Family VIII esterases present similarities to class C β‐lactamases, which show nucleophilic serines located at the S‐X‐X‐K motif instead of the G‐X‐S‐X‐G or G‐D‐S‐(L) motif shown by other carboxylesterase families. Indeed, the analysis of the substrate specificity revealed its capacity to hydrolyse nitrocefin as a model chromogenic cephalosporin substrate (40.4 ± 11.4 units·g−1), and a large battery of 66 structurally different esters (up to 1730 min−1), including bis(2‐hydroxyethyl)‐terephthalate (241.7 ± 8.5 units·g−1) and the mycotoxin T‐2 (1220 ± 52 units·g−1). It also showed acyltransferase activity through the synthesis of benzyl 3‐oxobutanoate (40.4 ± 11.4 units·g−1) from benzyl alcohol and vinyl acetoacetate.

Structural analyses of free and substrate‐bound forms of this homooctamer esterase suggest that EH7 presents a more opened and exposed S1 site having no steric hindrance for the entrance of substrates to the active site, more flexible R1, R2 and R3 regions allowing for the binding of a wide spectrum of substrates into the active site, and small residues in the conserved motif Y‐X‐X containing the catalytic Tyr enabling the entrance of large substrates. These unique structural elements in combination with docking experiments allowed us to gain valuable insights into the substrate specificity of this esterase and possible others belonging to family VIII.

>[4x]MHHHHHHHHHHLEVLFQGPSEFPMAQSNIIAGMDLNRLDRIAEHLDRAYLHPGKLAGTMTLVARRGEVVYCQAQGLRDVERQLPVERDTLFRIYSMTKPITSIALMQLYEQGRFLLDEPVHKYIPTWKNLRVYKTGSHPQMLTTAPQRPMTIRDLLTHQSGLTYGFMNRTNVDAAYRSLKLDGGPGHTLDRLIDELARLPLEFSPGTAWNYSVATDVCGYLVQLLSGMSLDDYFSKHIFQPLGMPDTFFTVPAEKLSRFAACYEYQPGDSFSLQDDPQGSAFAKAHGYLSGGGGLVSCVDDYYRFAQALANGGELDGARIIGRKTLEFMRMNHLPDNKGLPDVAIGSFSETPYDGTGFGLGFSVKLDVAKSQTVGSVGEYGWGGMASTNFFIDPEEDLLMVFMTQLIPSSTYAVRQELRAIINGALVDA> NYHSRSESTVENFLCRSACVFYTTYRNHGTDGDNFGYWVINTRQVAQLRRKLEMFTYARFDLELTFVITSTQEQSTIQGQDSPVLTHQIMYVPPGGPVPTKVNSYSWQTSTNPSVFWTEGSAPPRMSIPFISIGNAYSMFYDGWAKFDKQGTYGINTLNNMGTLYMRHVNDGSPGPIVSTVRIYFKPKHVKTWVPRPPRLCQYQKAGNVNFEPTGVTESRTDITTMQ;> RVRSITLGNSTITTQECANVVVGYGVWPTYLNDDEATAEDQPTQPDVATCRFYTLESVMWQQSSPGWWWKFPDALSNMGLFGQNMQYHYLGRAGYTVHVQCNASKFHQGCLLVVCVPEAEMGCATLANKPDQKSLSNGETANMFESQNSTGQTAVQANVINAGMGVGVGNLTIFPHQWINLRTNNSATIVMPYINSVPMDNMFRHNNFTLMIIPFAPLSYSTGATTYVPITVTVAPMCAEYNGLRLA;> GLPTMLTPGSNQFLTSDDFQSPSAMPQFDVTPEMDIPGQVNNLMEIAEVDSVVPVNNTEGKVLSIESYQIPVQSNSTNGSQVFGFPLMPGASSVLNRTLLGEILNYYTHWSGSIKLTFMFCGSAMATGKFLLAYSPPGAGAPTTRKEAMLGTHVIWDVGLQSSCVLCIPWISQTHYRYVVVDEYTAGGYITCWYQTNIVVPADTQSDCKILCFVSACNDFSVRMLKDTPFIKQDNFYQ

Coxsackie virus B5 (CVB5) is a member of Enterovirus-B (EV-B) species, which can cause various human diseases, such as viral encephalitis; herpangina; hand, foot, and mouth disease (HFMD); aseptic meningitis; and acute flaccid paralysis (1–3). Similar to other EV-B species, CVB5 is a nonenveloped, positive-sense single-strand RNA (+ssRNA) virus. P2, and P3 will break down into nonstructural proteins responsible for genome replication, whereas P1 is the precursor form of structural proteins VP1-VP4, which could be packaged into an icosahedral capsid. Here, we determined the atomic structures of CVB5 in three forms: mature full (F) particle (2.73 Å), intermediate altered (A) particle (2.81 Å), and procapsid empty (E) particle (2.95 Å).

The samples corresponding to both the bands were pooled and mixed for analysis by analytical ultracentrifugation (AUC), which suggested two types of particles–one containing RNA and the other lacking RNA with sedimentation coefficients of 143S and 80S, respectively. Compared with the map of the F particle, both maps of A and E particles had an expansion of ~4% with large openings on the 2-fold axes. The procapsid E particle and uncoating intermediate A particle of CVB5 were structurally almost indistinguishable, each with an expansion of ~4% in capsid radius, compared with the compact mature F particle, which is different from E3 and E30, whose procapsid E particles were comparable to the F particle but smaller than the A particle. However, no empty particle with a smaller radius was found after several rounds of 3D no-alignment classifications using different batches of particles, which is just like E18, CVB1 (13, 20). This is different from what has been found in the cases of E3, E30, E6, and E11, where an empty particle with a similar radius to the compacted F particle could be observed. We noted that the first seven residues of VP1 visualized on A particle would traverse the capsid and stop on the surface of the capsid, which was distinctive from the E particle where the corresponding residues were disordered, and all the other remaining residues were present on the interior of the capsid. But by analogy with other enteroviruses, the presence of pocket factor and myristoylistic acid in the mature F particle but not immature E particle and intermediate A particle, suggests that both the two molecules play important roles in the stabilization and integrity of mature virions for most of the EV-Bs.>[2x]EEEGRIRAMRAARSLGERTVTELILQHQNPQQLSSNLWAAVRARGCQFLGPAMQEEALKLVLLALEDGSALSRKVLVLFVVQRLEPRFPQASKTSIGHVVQLLYRASCFKVTKRDEDSS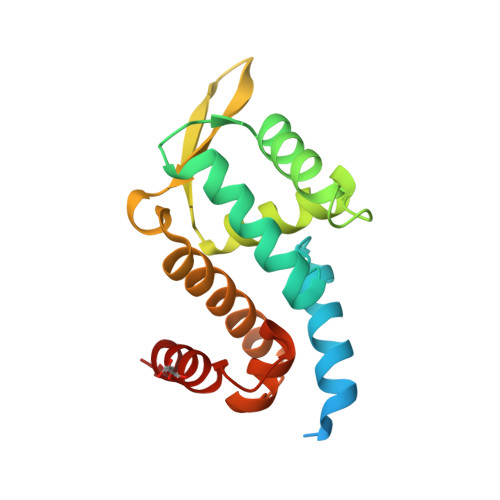LMQLKEEFRTYEALRREHDSQIVQIAMEAGLRIAPDQWSSLLYGDQSHKSHMQSIIDKLQT>ASPGVVISDDEPGYDLDLFCIPNHYAEDLERVFIPHGLIMDRTERLARDVMKEMGGHHIVALCVLKGGYKFFADLLDYIKALNRNSDRSIPMTVDFIRLKSYCNDQSTGDIKVIGGDDLSTLTGKNVLIVEDIIDTGKTMQTLLSLVRQYNPKMVKVASLLVKRTPRSVGYKPDFVGFEIPDKFVVGYALDYNEYFR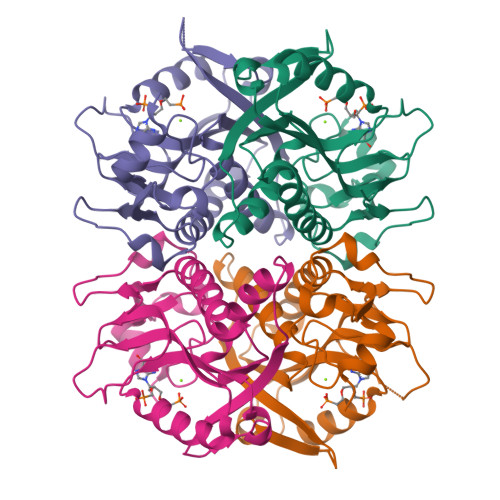DLNHVCVISETGKAKYKA[4x]> MN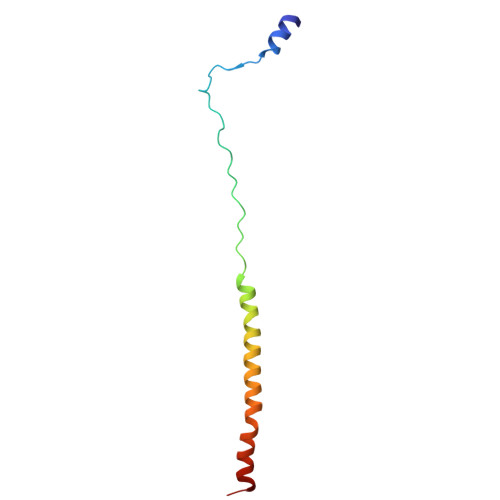VEELLRRIPLYNKYGKDFPQETVTRFQMPEFKLPALQPTRDLLCPWYEECDNITKVCQLHDSSNKKFDQWYKEQYLS> MSVTIDHTTENAAPAQAPVSDRAWALFRALDGKGLVPDGYVEGWKKTFEEDFSPRRGAELVARAWTDPEFRQLLLTDGTAAVAQYGYLGPQGEYIVAVEDTPTLKNVIVCSLCSCTAWPILGLPPTWYKSFEYRARVVREPRKVLSEMGTEIASDIEIRV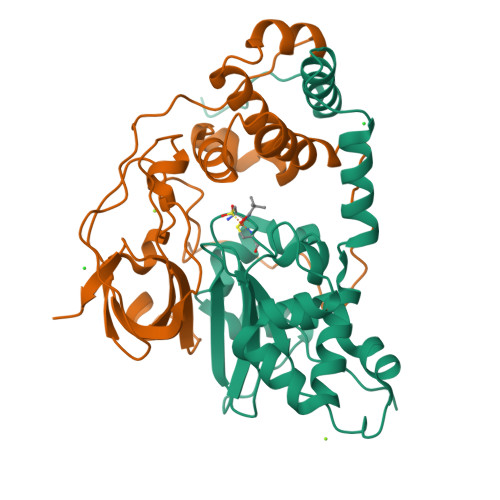YDTTAETRYMVLPQRPAGTEGWSQEQLQEIVTKDCLIGVAIPQVPTV;> MDGVHDLAGVQGFGKVPHTVNADIGPTFHAEWEHLPYSLMFAGVAELGAFSVDEVKYVVERMEPRHYMMTPYYERYVIGVATLMVEKGILTQDELESLAGGPFPLSRPSESEGRPAPVETTTFEVGQRVRVRDEYVPGHIRMPAYCRGRVGTISHRTTEKWPFPDAIGHGRNDAGEEPTYHVKFAAEELFGSDTDGGSVVVDLFEGYLEPAA>XELKAIAQEF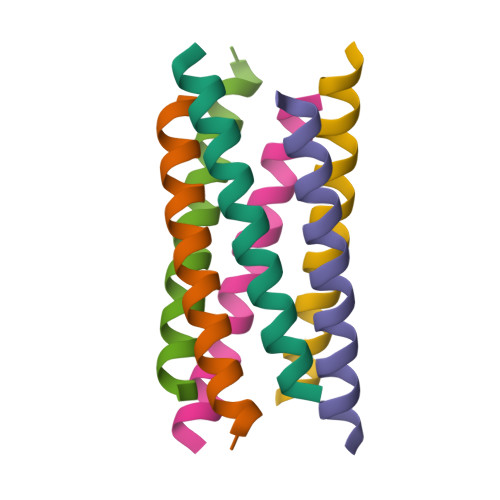KAIAKEFKAIAWEFKAIAQKX[3x]(2~{E},4~{E},6~{E},8~{E})-3,7-dimethyl-9-(2,6,6-trimethylcyclohexen-1-yl)nona-2,4,6,8-tetraen-1-amine 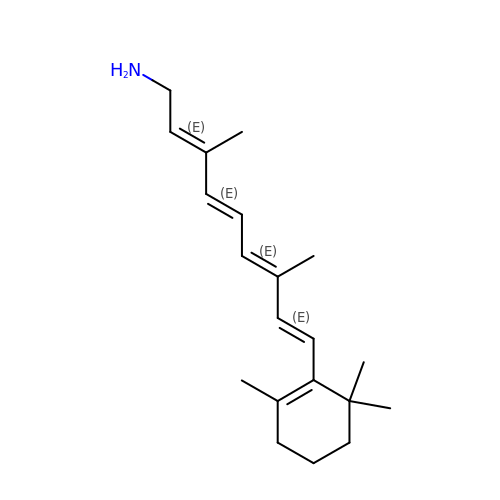| C20 H31 N | ILYSIVSSNXQZQG-OVSJKPMPSA-N> QDTSPDTLVVTANRFEQPRSTVLAPTTVVTRQDIDRWQSTSVNDVLRRLPGVDITQNGGSGQLSSIFIRGTNASHVLVLIDGV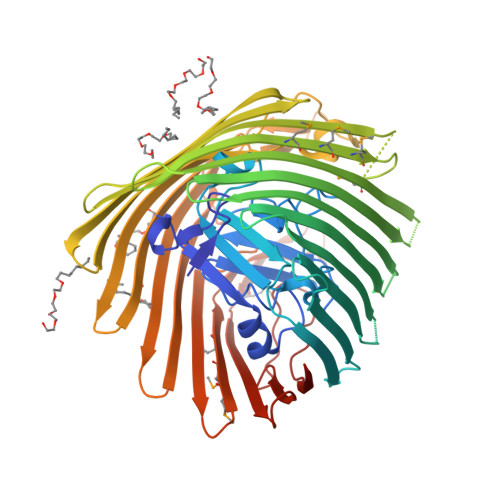RLNLAGVSGSADLSQFPIALVQRVEYIRGPRSAVYGSDAIGGVVNIITTRDEPGTEISAGWGSNSYQNYDVSTQQQLGDKTRVTLLGDYAHTHGYDVVAYGNTGTQAQTDNDGFLSKTLYGALEHNFTDAWSGFVRGYGYDNRTNYDAYYSPGSPLLDTRKLYSQSWDAGLRYNGELIKSQLITSYSHSKDYNYDPHYGRYDSSATLDEMKQYTVQWANNVIVGHGSIGAGVDMQMQMTTPGTGYVEDGYDQRNTGIYLTGLQQVGDFTFEGAARSDDNSQFGRHGTWQTSAGWEFIEGYRFIASYGTSYKAPNLGQLYGFYGNPNLDPEKSKQWEGAFEGLTAGVNWRISGYRNDVSDLIDYDDHTLKYYNEGKARIKGVEATANFDTGPLTHTVSYDYVDARNAITDTPLLRRAKQQVKYQLDWQLYDFDMGMTMQYLGTRYDKDYSSYPYQTVKMGGVSLWDLAVAYPVTSHLTVRGKIANLFDKDYETVYGYQTAGREYTLSGSYTF8-Oxoguanine (GO) is a major purine oxidation product in DNA. The major way to remove GO is the base excision repair pathway, usually initiated by a GO-DNA glycosylase. While no enzymes with an A/G specific-DNA glycosylase or a dGOTPase activity have been discovered in these species, a GO-DNA glycosylase called AGOG (for Archaeal GO-DNA Glycosylase) has been initially identified in the hyperthermophilic archaeon Pyrobaculum aerophilum. Despite very low sequence identity, AGOG is structurally similar to eukaryotic and prokaryotic OGG1 and OGG2 GO-DNA glycosylases and, like these two proteins, belongs to the Endo III structural superfamily partly defined by the central helix-hairpin-helix (HhH) element followed by a glycine/proline-rich region and an aspartate (GPD).

Tga-AGOG has an extension of 11 or 19 residues at the N-terminus compared to Pae-AGOG or Pab-AGOG, respectively. This non-structured part of the protein was cleaved between residues R8-I9 by trypsin and the first residue that could be located without ambiguity in the electron density map was Y11 (Trypsin was used to remove the His-Tag because the internal proteolytic site between the Tag and the N-terminus of Tga-AGOG is thrombin resistant). Another part of Tga-AGOG appears to be more flexible than in Pab- and Pae-AGOG. In the two molecules present in the asymmetric unit, residues between L236 and G240 were not clearly visible and were not assigned due to high mobility. In fact, the mean b-factor for the N/C domain (43 Å2) is almost twice as high as that observed for the HhH domain (23 Å2). This observation could be related to the absence of a disulfide bridge between the two cysteine residues present in Tga-AGOG (C32 and C250, hypothetical S/S in Supplementary Figure S5A), despite the fact that they are close to each other in the 3D structure (3.54 Å). Despite differences in the number of disulphide bridges, Tga-AGOG adopts the same conformation as Pab- or Pae-AGOG with minor differences located mainly in the N/C domain. Under the same conditions, the oxidized and reduced forms of Tga-AGOG are indistinguishable in terms of their activity (at least up to 80°C), indicating that this enzyme, like Pab-AGOG, does not rely on disulphide bridges and instead achieves heat resistance by means that are insensitive to a reducing agent. The sequence alignment based on 3D structures unambiguously shows that the catalytic lysine is strictly conserved in AGOGs and corresponds to K142 and K162 of Pab-AGOG and Tga-AGOG, respectively.

>[2x]GSHMTLDRFVRIKYREDNEKVNRLVEILRELGLDCARTIEEKVDLQFDALRNLRENLKDDELFIKLVIANALVSYQLSGKGEDWWWEFSRYFSENPPEDIVEAYSSFLPNSKTNRRLVAGKLKRIERVEPFLSPLSISEIRDYYFNGMERLRDELARVMKAKRSAKTIVFAVKMFGYAGRIAFSAFVPYPMAIEIPDDVRINAYTKRFTSEPPVSFWGRIAEETGIPPLHIDSILWPVLGGKGEVLRRLKKHCGEKAERILELRDL> KDPKRLYCKNGGFFLRIHPDGRVDGVREKSDPHIKLQLQAEERGVVSIKGVCANRYLAMKEDGRLLASKCVTDECFFFERLESNNYNTYRSRKYTSWYVALKRTGQYKLGSK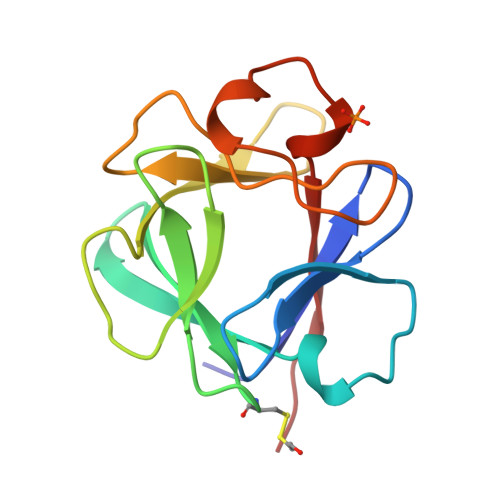TGPGQKAILFLPMSAKS>AQQNILSVHILNQQTGKPAADVTVTLEKKADNGWLQLNTAKTDKDGRIKALWPEQTATTGDYR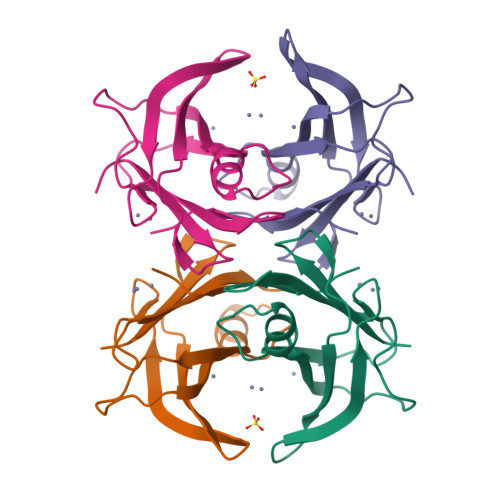VVFKTGDYFKKQNLESFFPEIPVEFHINKVNEHYHVPLLLSQYGYSTYRGS[4x]>GKKMMTTDGNTATAHVAYAMSEVAAIYPITPSSTMGEEADDWAAQGRKNIFGQTLTIREMQSEAGAAGAVHGALAAGALTTTFTASQGLLLMIPNMYKISGELLPGVFHVTARAIAAHALSIFGDHQDIYAARQTGFAMLASSSVQEAHDMALVAHLAAIESNVPFMHFFDGFRTSHEIQKIEVLDYADMASLVNQKALAEFRAKSMNPEHPHVRGTAQNPDIYFQGREAANPYYLKVPGIVAEYMQKVASLTGRSYKLFDYVGAPDAERVIVSMGSSCETIEEVINHLAAKGEKIGLIKVRLYRPFVSEAFFAALPASAKVITVLDRTKEPGAPGDPLYLDVCSAFVERGEAMPKILAGRYGLGSKEFSPAMVKSVYDNMSGAKKNHFTVGIEDDVTGTSLPVDNAFADTTPKGTIQCQFWGLGADGTVGANKQAIKIIGDNTDLFAQGYFSYDSKKSGGITISHLRFGEKPIQSTYLVNRADYVACHNPAYVGIYDILEGIKDGGTFVLNSPWSSLEDMDKHLPSGIKRTIANKKLKFYNIDAVKIATDVGLGGRINMIMQTAFFKLAGVLPFEKAVDLLKKSIHKAYGKKGEKIVKMNTDAVDQAVTSLQEFKYPDSWKDAPAETKAEPMTNEFFKNVVKPILTQQGDKLPVSAFEADGRFPLGTSQFEKRGVAINVPQWVPENCIQCNQCAFVCPHSAILPVLAKEEELVGAPANFTALEAKGKELKGYKFRIQINTLDCMGCGNCADICPPKEKALVMQPLDTQRDAQVPNLEYAARIPVKSEVLPRDSLKGSQFQEPLMEFSGACSGCGETPYVRVITQLFGERMFIANATGCSSIWGASAPSMPYKTNRLGQGPAWGNSLFEDAAEYGFGMNMSMFARRTHLADLAAKALESDASGDVKEALQGWLAGKNDPIKSKEYGDKLKKLLAGQKDGLLGQIAAMSDLYTKKSVWIFGGDGWAYDIGYGGLDHVLASGEDVNVFVMDTEVYSNTGGQSSKATPTGAVAKFAAAGKRTGKKDLARMVMTYGYVYVATVSMGYSKQQFLKVLKEAESFPGPSLVIAYATCINQGLRKGMGKSQDVMNTAVKSGYWPLFRYDPRL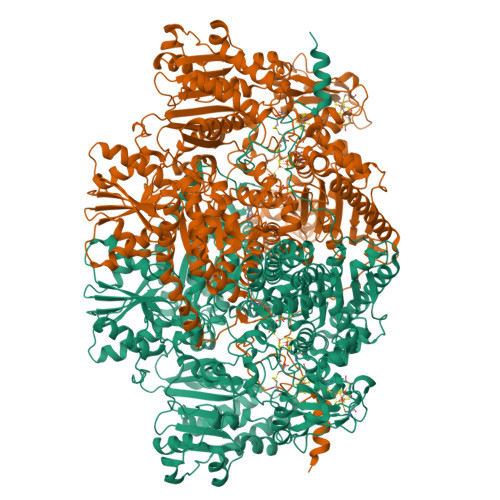AAQGKNPFQLDSKAPDGSVEEFLMAQNRFAVLDRSFPEDAKRLRAQVAHELDVRFKELEHMAATNIFESFAPAGGKADGSVDFGEGAEFCTRDDTPMMARPDSGEACDQNRAGTSEQQGDLSKRTKK[2x]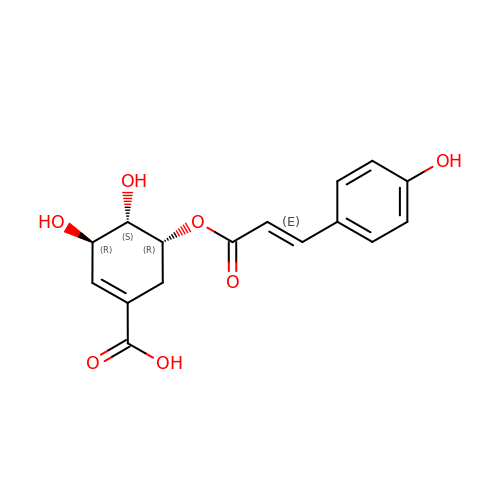(3R,4S,5R)-3,4-dihydroxy-5-{[(2E)-3-(4-hydroxyphenyl)prop-2-enoyl]oxy}cyclohex-1-ene-1-carboxylic acid | C16 H16 O7 | GVECSFFLZYNEBO-ADMZAUMBSA-N2-(5-chloro-2-methyl-1H-indol-3-yl)ethan-1-amine | C11 H13 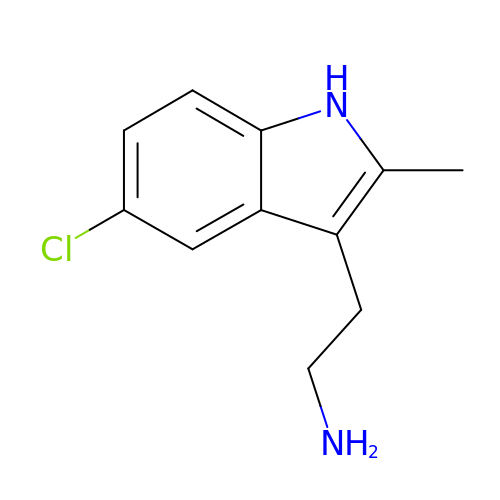Cl N2 | PPPQHAMKVHECAL-UHFFFAOYSA-N(4-{[(4-{[AMINO(IMINO)METHYL]AMINO}BUTYL)AMINO]METHYL}-5-HYDROXY-6-METHYLPYRIDIN-3-YL)METHYL DIHYDROGEN PHOSPHATE 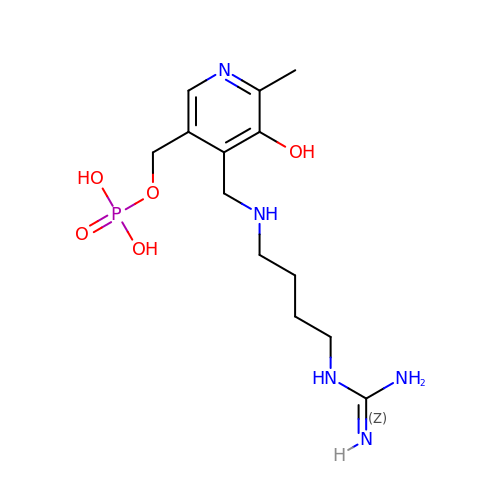| C13 H24 N5 O5 P | SIKJBFNFPRPKQR-UHFFFAOYSA-N GDP-N-acetylperosamine-coenzyme A | C39 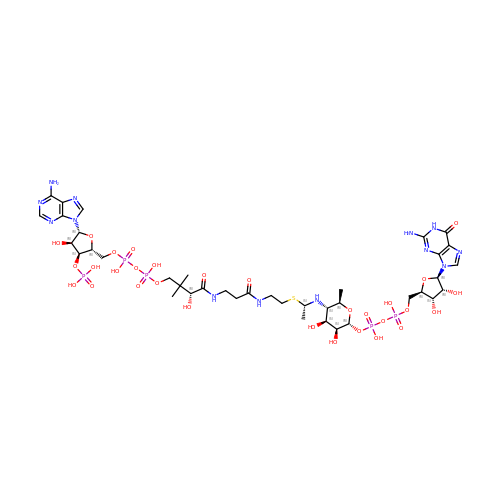H64 N13 O30 P5 S | JPJUGYYIHUXJRE-NLBQBQJKSA-N>[4x]MNDNVAWFKQAKYGMMIHWGLYSLLAGEYRGESSSAYAEWIQSKFQIPNAEYGNLATAFNPLYFDAKKIVALAKQCGMQYL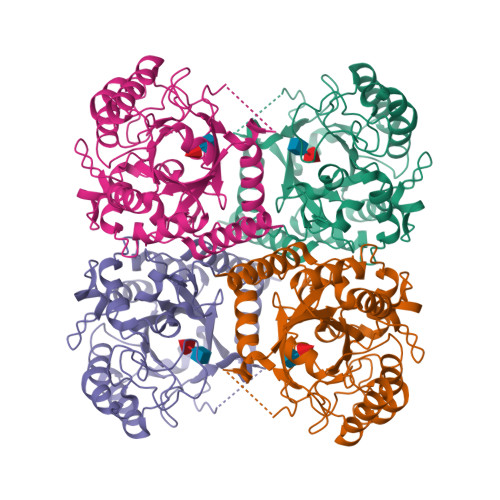VVTTKHHDGFAMYHSKVDAYNVYDATPFHRDIIGELAEACQKAGLKFGLYYSQDLDWHDPNGGGYKSNDVETAGTTWDNSWDFPDEDQKNFDLCFDNKILPQIKEIMSNYGDIATAWFAVPMTLSEAQSQTIYDTVRELQPNCLINSRLGNGKYDFVSLGDNEIPKNKEDMNKTDVDYNEITGFKPSPLGLYETAGTINDSWGFSYHDQNWKTPRTLYRYKQHLNDFGINYLLNVGLDPLGRVPMMAEENLLAAKALEDEANRL>[4x]APVRSLNCTLRDSQQKSLVMSGPYELKALHLQGQDMEQQVVFSMSFVQGEESNDKIPVALGLKEKNLYLSCVLKDDK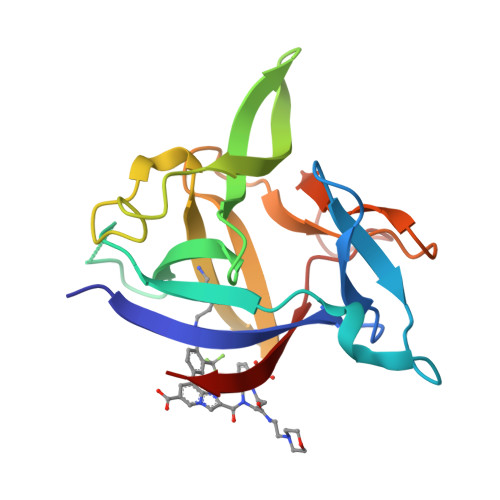PTLQLESVDPKNYPKKKMEKRFVFNKIEINNKLEFESAQFPNWYISTSQAENMPVFLGGTKGGQDITDFTMQFVSS> MTEFWLISAPGEK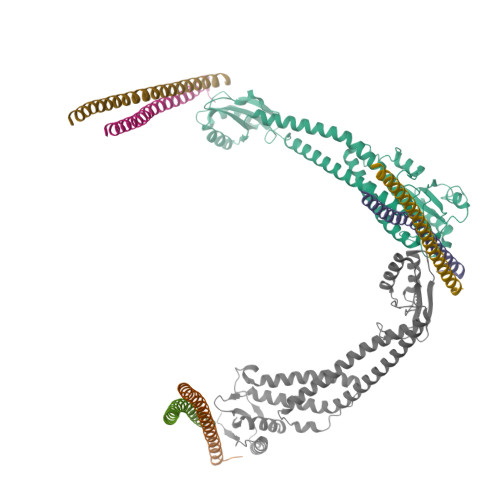TCQQTWEKLHAATTKNNNLAVSSKFNIPDLKVGTLDVLVGLSDELAKLDAFVEGVVKKVAQYMADVLEDSKDKVQENLLASGVDLVTYITRFQWDMAKYPIKQSLKNISEIIAKGVTQIDNDLKSRASAYNNLKGNLQNLERKNAGSLLTRSLAEIVKKDDFVLDSEYLVTLLVVVPKLNHNDWIKQYETLAEMVVPRSSNVLSEDQDSYLCNVTLFKKAVDDFRHKARENKFIVRDFQYNEEEMRADKEEMNRLSTDKKKQFGPLVRWLKVNFSEAFIAWIHIKALRVFVESVLRYGLPVNFQAMLLQPNKKSVKKLREVLHELYKHLDSSAAAIIDAPMDIPGLNLSQQEYYPYVYYKIDCNLLEFK;>[3x]MALSDADVQKQIKHMMAFIEQEANEKAEEIDAKAEEEFNIEKGRLVQTQRLKIMEYYEKKEKQIEQQKKIQMSNLMNQARLKVLRARDDLITDLLNEAKQRLSKVVKDTTRYQVLLDGLVLQGLYQLLEPRMIVRCRKQDFPLVKAAVQKAIPMYKIATKKDVDVQIDLEAYLPEDIAGGVEIYNGDRKIKVSNTLESRLDLIAQQMMPEVRGALFGANANRKFLD;>MASQSQGIQQLLQAEKRAAEKVADARKRKARRLKQAKEEAQMEVEQYRREREQEFQSKQQAAMGSQGNLSAEVEQATRRQVQGMQSSQQRNRERVLTQLLGMVCDVRPQVHPNYRITV[3x];> MGELFRSEEMTLAQLFLQSEAAYCCVSELEELGKVQFRDLNPDVNVFQRKFVNEVRRCEEMDRKLRFVEKEIRKANIPIMDTGENPEVPFPRDMIDLEANFEKIENELKEINTNQEALKRNFLELTELKFILRKTQQFFDEMADPDLLEESSSLLEPNEMGRGAPLRLGFVAGVINRERIPTFERMLWRVCRGNVFLRQAEIENPLEDPVTGDYVHKSVFIIFFQGDQLKNRVKKICEGFRASLYPCPETPQERKEMASGVNTRIDDLQMVLNQTEDHRQRVLQAAAKNIRVWFIKVRKMKAIYHTLNLCNIDVTQKCLIAEVWCPVTDLDSIQFALRRGTEHSGSTVPSILNRMQTNQTPPTYNKTNKFTHGFQNIVDAYGIGTYREINPAPYTVITFPFLFAVMFGDFGHGILMTLFAVWMVLRESRILSQKNENEMFSMVFSGRYIILLMGLFSIYTGLIYNDCFSKSLNIFGSSWSVRPMFTIGNWTEETLLGSSVLQLNPAIPGVFGGPYPFGIDPIWNIATNKLTFLNSFKMKMSVILGIIHMLFGVSLSLFNHIYFKKPLNIYFGFIPEIIFMSSLFGYLVILIFYKWTAYDAHSSRNAPSLLIHFINMFLFSYPESGNAMLYSGQKGIQCFLIVVAMLCVPWMLLFKPLILRHQYLRKKHLGTLNFGGIRVGNGPTEEDAEIIQHDQLSTHSEDAEEPTEDEVFDFGDTMVHQAIHTIEYCLGCISNTASYLRLWALSLAHAQLSEVLWTMVIHIGLHVRSLAGGLGLFFIFAAFATLTVAILLIMEGLSAFLHALRLHWVEFQNKFYTGTGFKFLPFSFEHIREGKFDE> GSHMKNSVSVDLPGSMKVLVSKSSNADGKYDLIATVDALELSGTSDKNNGSGVLEGVKADASKVKLTISDDLGQTTLEVFKSDGSTLVSKKVTSKDKSSGEEKFNEKGEVSEKIITRADGTRLEYTGIKSDGSGKAKEVLKGYVL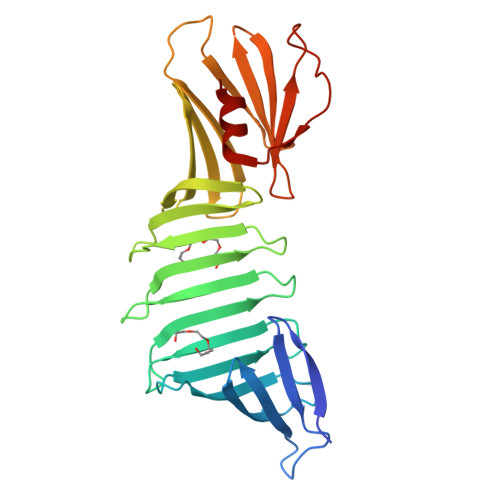EGTLTAEKTTLVVKEGTVTLSKNISKSGAVSVELNDTDSSAATKKTAAWNSGTSTLTITVNSKKTKDLVFTSSNTITVQQYDSNGTSLEGSAVEITKLDEIKNALK Undecaprenyl pyrophosphate synthase is a cis-prenyl transferase and is responsible for the condensation of eight molecules of IPP with farnesyl diphosphate to form the C55 species, undecaprenyl diphosphate. Following the condensation, undecaprenyl diphosphate is converted to Lipid I, Lipid II, and lastly, to bacterial cell wall peptidoglycans. The catalytic site is composed of four binding pockets, and it is responsible for accommodating the large substrates, FPP and IPP, and for transferring the phosphate groups and metal ions between the two substrates during the condensation reaction. Comparison of these crystal structures reveals that UPPS is a highly flexible protein system, showing very mobile binding pockets in the active site region.

In addition, we have crystallized E. coli UPPS with the flexible loop to further investigate the large pocket-size fluctuation in our MD simulations. To help confirm the nature of this pocket closure on ligand removal (or expansion on ligand binding), we crystallized the E. coli UPPS in the ligand-free form. Crystal structures of the ligand-bound and apo form of UPPS reveal that a major pocket closure occurs upon ligand removal, from 1032 to 432 Å3 and is in good agreement with the time-averaged pocket volume (332 Å3) of the apo form obtained from the MD simulation. We also described the first complete apo E. coli UPPS structure with an intact active site. We observed an excellent agreement between the calculated average pocket volume from the apo enzyme simulation and the newly solved crystal structure. Furthermore, it appears that the active site of the apo structure opens and expands considerably upon binding of bisphosphonate ligands, shifting the population of UPPS enzymes to a markedly different conformation. The most dynamic region of UPPS is the loop comprising residues 72–82.

>[2x]MMLSATQPLSEKLPAHGCRHVAIIMDGNGRWAKKQGKIRAFGHKAGAKSVRRAVSFAANNGIEALTLYAFSSENWNRPAQEVSALMELFVWALDSEVKSLHRHNVRLRIIGDTSRFNSRLQERIRKSEALTAGNTGLTLNIAANYGGRWDIVQGVRQLAEKVQQGNLQPDQIDEEMLNQHVCMHELAPVDLVIRTGGEHRISNFLLWQIAYAELYFTDVLWPDFDEQDFEGALNAFANRERRFGGTEPGDETA> GDEREDDGVPSAAYVTQLYYKISRIDWDYEVEPARIKGIHYGPDIA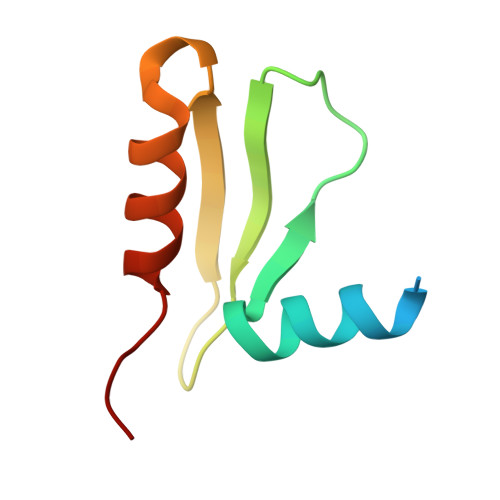QPINMDSSHHSRCFISDYLWSLVPTAW N-[2-(5-methoxy-2-phenyl-1H-indol-3-yl)ethyl]acetamide | C19 H20 N2 O2 | 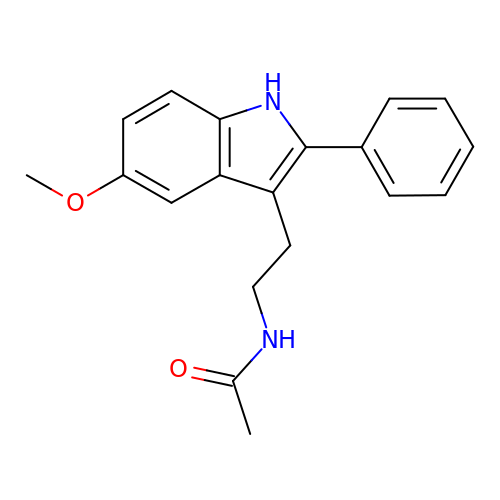OFCLARYYBGKCHN-UHFFFAOYSA-N YP_001813558.1 and its homologs (dimeric dUTPases, MazG proteins and HisE-encoded phosphoribosyl ATP pyrophosphohydrolases) form a superfamily of all-α-helical NTP pyrophosphatases. The α-helical NTP pyrophos­phatases share a highly conserved four-helix bundle, one face of which forms the active site, while the other participates in oligomer assembly. Nucleoside triphosphate pyrophosphatases (or pyrophospho­hydrolases; NTPases) perform the important function of hydrolyzing the α–β phosphodiester bond of nucleoside triphosphates (NTPs) and are often involved in removing noncanonical nucleotide triphos­phates to prevent their incorporation into DNA or RNA. dUTP pyrophosphatase (dUTPase; EC 3.6.1.23) catalyzes the hydrolysis of dUTP to dUMP and pyrophosphate. Here, we report the crystal structure of NTPase YP_001813558.1 from the extremophile Exiguobacterium sibiricum 255-15 (PF09934, DUF2166), which was originally isolated from the Siberian permafrost.

The crystal structure of a putative NTPase, YP_001813558.1 from Exiguo­bacterium sibiricum 255-15 (PF09934, DUF2166) was determined to 1.78 Å resolution. However, in YP_001813558.1, an unexpected intertwined swapping of two of the helices that compose the conserved helix bundle results in a ‘linked dimer’ that has not previously been observed for this family. The structure reveals an interesting variant of the all-α-helical NTP pyrophosphatase fold family that contains an unusual intertwined swapping of helical segments, resulting in an obligatory dimer that cannot dissociate without unfolding of the monomers. This novel ‘linked dimer’ defines a new subfamily of the α-helical NTP pyrophosphatase fold and is distinct from other previously observed domain-swapped dimers. Size-exclusion chromatography combined with static light scattering confirmed that the dimer is the major oligomeric state in solution. A surface area of 5104 Å2 per monomer is buried upon dimer formation. Divalent cations, preferably magnesium, are essential for NTPase activity. Interestingly, although the YP_001813558.1 active site assembles quite differently from those of the other NTPases, the putative metal-binding sites in all three proteins are absolutely conserved, except for a one-residue offset of Asp95 in YP_001813558.1. Furthermore, the active-site residues that are involved in sugar binding of the NTPs are also conserved when compared with other α-helical NTPases, but those that recognize the nucleotide bases are not conserved, suggesting a different substrate specificity. The corresponding residues in YP_001813558.1 are Val10, His14 and His19; His14 N∊2 is hydrogen bonded to the O2 atom of a 1,2-ethanediol molecule in the ligand-binding site. The corresponding pyrophosphate-recognition loop in YP_001813558.1 is located between H5 and H6.

> GMKQPNYYQDVKQFHQTFHHPGADQPTAIPLDRGVKRATWTAEEAVVEFLHQSSQNETEFLAAIETFKAGLDQAVKKSLKETYPVTEVERLVGQGDALTDALYFIMGSFVEAGLEPGPLFEIVQQANMAKLGPDGQPIFRESDQKVMKPDGWLPPEPQLEAEVVRQMKEKA> MSDGTSQPDSGNAVHSAARVERAADGPGGSGGGGSGGGGVGVSTGSYDNQTHYRFLGDGWVEITALATRLVHLNMPKSENYCRIRVHNTTDTSVKGNMAKDDAHEQIWTPWSLVDANAWGVWLQPSDWQYICNTMSQLNLVSLDQEIFNVVLKTVTEQDLGGQAIKIYNNDLTACMMVAVDSNNILPYTPAANSMETLGFYPWKPTIASPYRYY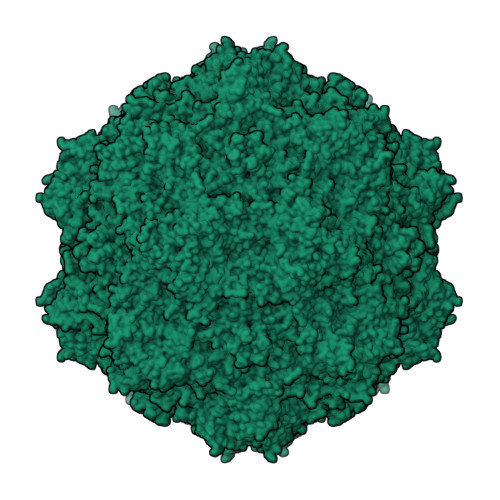FCVDRDLSVTYENQEGTVEHNVMGTPKGMNSQFFTIENTQQITLLRTGDEFATGTYYFDTNPVKLTHTWQTNRQLGQPPLLSTFPEADTDAGTLTAQGSRHGTTQMGVNWVSEAIRTRPAQVGFCQPHNDFEASRAGPFAAPKVPADITQGVDKEANGSVRYSYGKQHGENWASHGPAPERYTWDETSFGSGRDTKDGFIQSAPLVVPPPLNGILTNANPIGTKNDIHFSNVFNSYGPLTAFSHPSPVYPQGQIWDKELDLEHKPRLHITAPFVCKNNAPGQMLVRLGPNLTDQYDPNGATLSRIVTYGTFFWKGKLTMRAKLRANTTWNPVYQVSAEDNGNSYMSVTKWLPTATGNMQSVPLITRPVARNTY6-amino-2-(methylamino)-4-(2-{[(3S,5S,7S)-tricyclo[3.3.1.1~3,7~]dec-1-ylmethyl]amino}ethyl)-1,7-dihydro-8H-imidazo[4,5-g]quinazolin-8-one 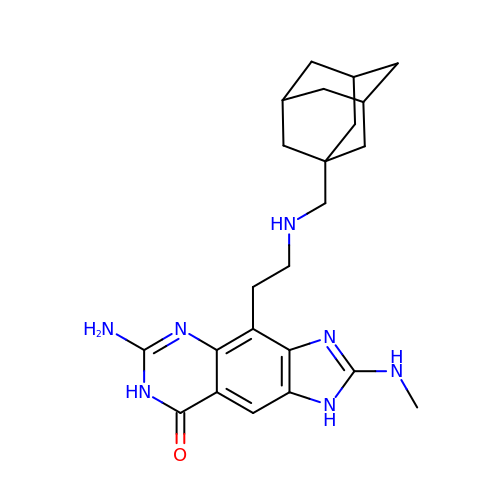| C23 H31 N7 O | HJDZMDZEUQKVPL-CAUGRDAOSA-N3-{[4-amino-1-(1-methylethyl)-1H-pyrazolo[3,4-d]pyrimidin-3-yl]ethynyl}phenol | C16 H15 N5 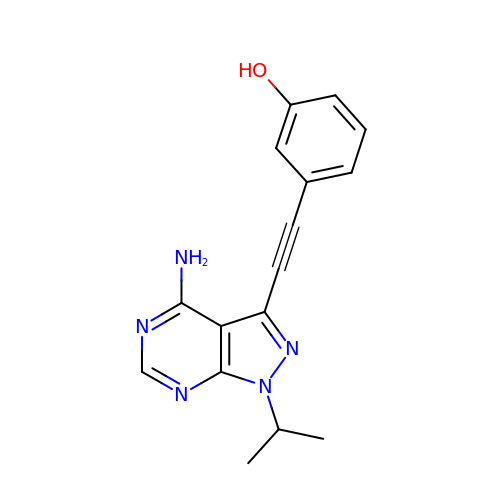O | HFGDXJQGICLTIE-UHFFFAOYSA-N>[2x]MTSEHRSASVTPRHI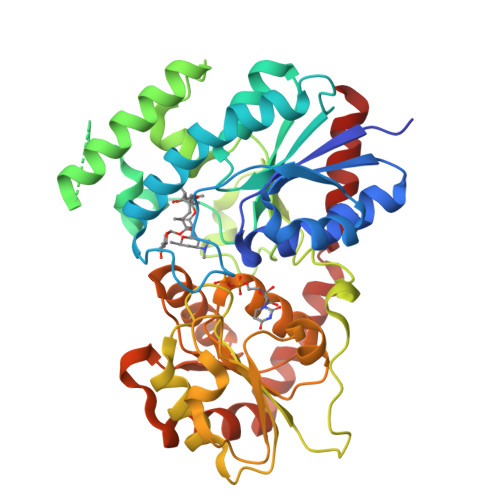SFFNIPGHGHVNPSLGIVQELVARGHRVSYAITDEFAAQVKAAGATPVVYDSILPKESNPEESWPEDQESAMGLFLDEAVRVLPQLEDAYADDRPDLIVYDIASWPAPVLGRKWDIPFVQLSPTFVAYEGFEEDVPAVQDPTADRGEEAAAPAGTGDAEEGAEAEDGLVRFFTRLSAFLEEHGVDTPATEFLIAPNRCIVALPRTFQIKGDTVGDNYTFVGPTYGDRSHQGTWEGPGDGRPVLLIALGSAFTDHLDFYRTCLSAVDGLDWHVVLSVGRFVDPADLGEVPPNVEVHQWVPQLDILTKASAFITHAGMGSTMEALSNAVPMVAVPQIAEQTMNAERIVELGLGRHIPRDQVTAEKLREAVLAVASDPGVAERLAAVRQEIREAGGARAAADILEGILAEAG5-[(3,4-dimethoxyphenyl)methyl]pyrimidine-2,4-diamine 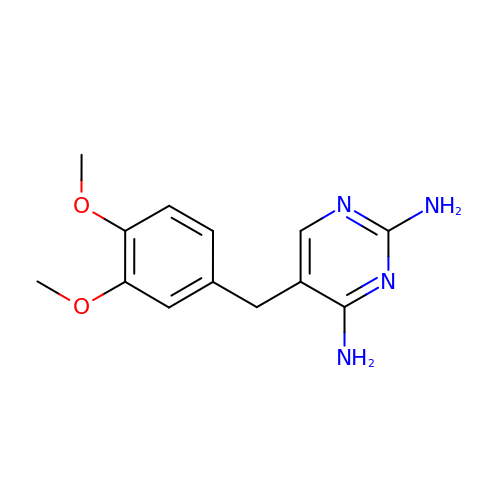| C13 H16 N4 O2 | LDBTVAXGKYIFHO-UHFFFAOYSA-N[1,1'-biphenyl]-4,4'-disulfonic 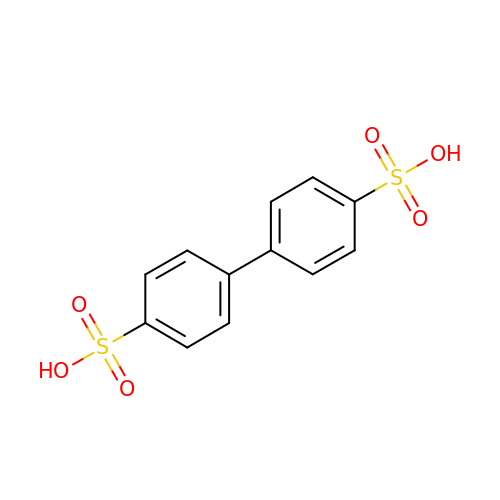acid | C12 H10 O6 S2 | ABSXMLODUTXQDJ-UHFFFAOYSA-N>[8x]GPGSMTAELENKVAIITGACGGIGLETSRVLARAGARVVLADLPETDLAGAAASVGRGAVHHVVDLTNEVSVRALIDFTIDTFGRLDIVDNNAAHSDPADMLVTQMTVDVWDDTFTVNARGTMLM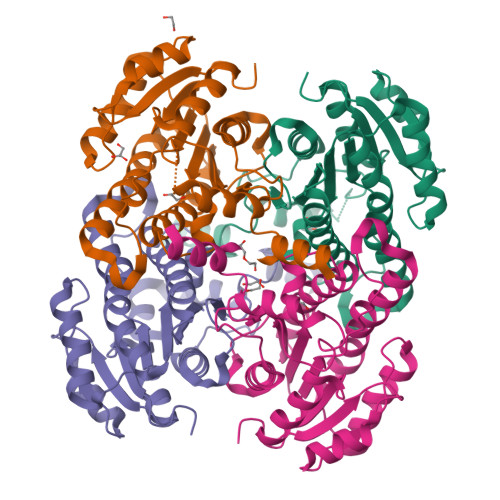CKYAIPRLISAGGGAIVNISSATAHAAYDMSTAYACTKAAIETLTRYVATQYGRHGVRCNAIAPGLVRTPRLEVGLPQPIVDIFATHHLAGRIGEPHEIAELVCFLASDRAAFITGQVIAADSGLLAHLPGLPQIRASVAELQSQP>YVDYKDDDDKEFEEVSEYCSHMIGSGHLQSLQRLIDSQMETSSQITFEFVDQEQLKDPVCYLKKAFLLVQDIMEDTMRFRDNTPNAIAIVQLQELSLRLKSCFTKDYEEHDKACVRTFYETPLQLLEKVKNVFNETKNLLDKDWNIFSKNCNNSFA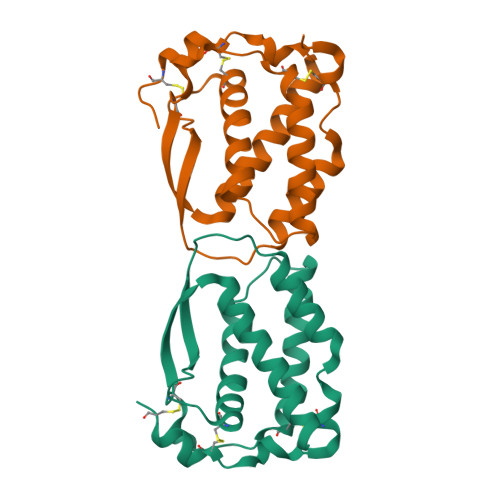ECSSQGHERQSEGSPRHHHHHHAAAN[2x]> MEAEPPLYPMAGAAGPQGDEDLLGVPDGPEAPLDELVGAYPNYNEEEEERRYYRRKRLGVLKNVLAASAGGMLTYGVYLGLLQMQLILHYDETYREVKYGNMGLPDIDSKMLMGINVTPIAALLYTPVLIRFFGTKWMMFLAVGIYALFVSTNYWERYYTLVPSAVALGMAIVPLWASMGNYITRMAQKYHEYSHYKEQDGQGMKQRPPRGSHAPYLLVFQAIFYSFFHLSFACAQLPMIYFLNHYLYDLNHTLYNVQSCGTNSHGILSGFNKTVLRTLPRSGNLIVVESVLMAVAFLAMLLVLGLCGAAYRPTEEIDLRSVGWGNIFQLPFKHVRDYRLRHLVPFFIYSGFEVLFACTGIALGYGVCSVGL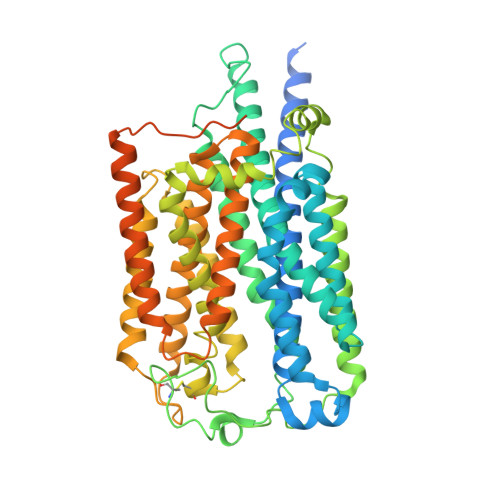ERLAYLLVAYSLGASAASLLGLLGLWLPRPVPLVAGAGVHLLLTFILFFWAPVPRVLQHSWILYVAAALWGVGSALNKTGLSTLLGILYEDKERQDFIFTIYHWWQAVAIFTVYLGSSLHMKAKLAVLLVTLVAAAVSYLRMEQKLRRGVAPRQPRIPRPQHKVRGYRYLEEDNSDESDAEGEHGDGAEEEAPPAGPRPGPEPAGLGRRPCPYEQAQGGDGPEEQ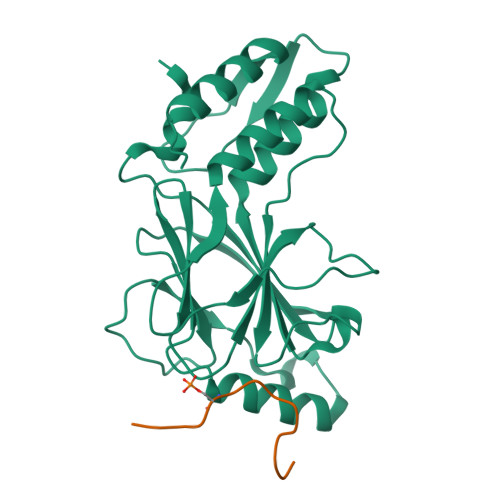>SEFENPLKRLLVPGEEWEFEVTAFYRGRQVFQQTISCPEGLRLVGSEVGDRTLPGWPVTLPDPGMSLTDRGVMSYVRHVLSCLGGGLALWRAGQWLWAQRLGHCHTYWAVSEELLPNSGHGPDGEVPKDKEGGVFDLGPFIVDLITFTEGSGRSPRYALWFCVGESWPQDQPWTKRLVMVKVVPTCLRALVEMARVGGASSLENTVDLHISNSHPLSLTSDQYKAYLQDLVEGMDFQGPGES[2x];>[2x]SGCFEDLAISASTSLGWG> MSAILKRAAKYKRVSSILCEGEAHLRDPFTPPPVILKPPAPRKDKKPDDITDFPAQKLIPLPESIPYQEGKYRPASIPMVAGFFPYNCYLQQGKVYSWCSCGI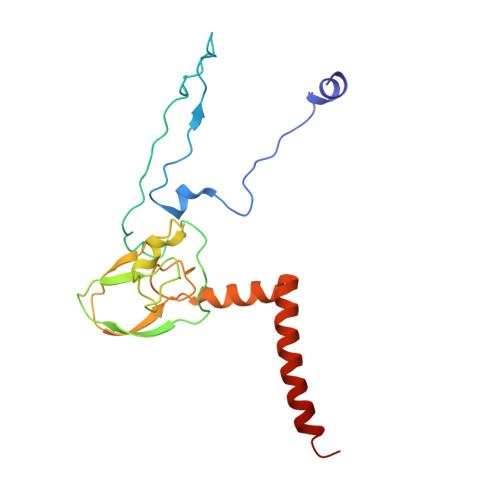SQSGPWCDGLCNSVVTRCRPVVFNVSQSGYYKICNCKFSANAPFCNNTHRKMVRYHHQTHRGFYEIWGAALFVLGWVYMGFNYYT(2Z,6E)-3,7,11-trimethyldodeca-2,6,10-trien-1-ol | 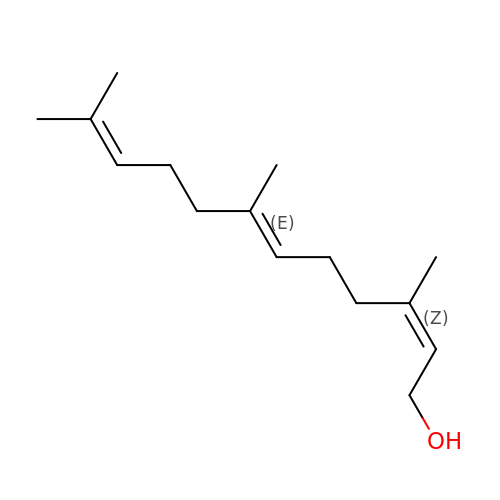C15 H26 O | CRDAMVZIKSXKFV-PVMFERMNSA-N2-[[1-methoxy-4-oxidanyl-7-(4-phenylphenoxy)isoquinolin-3-yl]carbonylamino]ethanoic acid | C25 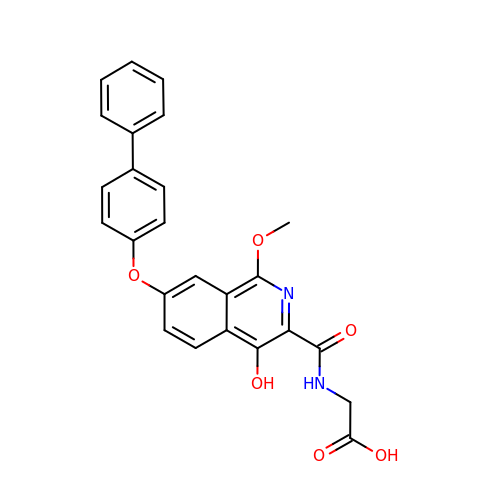H20 N2 O6 | ORXLENKYLYVGFT-UHFFFAOYSA-N>[4x]AVTGQVDVKLNISTGCTVGGSQTEGNMNKFGTLNFGKTSGTWNNVLTAEVASAATGGNISVTCDGTDPVDFTVAIDGGERTDRTLKNTASADVVAYNVYRDAARTNLYVVNQPQQFTTVS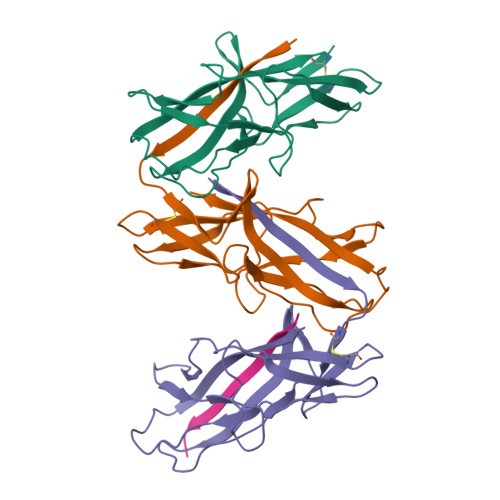GQATAVPIFGAIAPNTGTPKAQGDYKDTLLVTVNF> SAPAAALKKAAEAAEPATVTEDATDLQNEVDQELLKDMYGKEHVNIVFIGHVDAGKSTLGGNILFLTGMVDKRTMEKIEREAKEAGKESWYLSWALDSTSEEREKGKTVEVGRAYFETEHRRFSLLDAPGHKGYVTNMINGASQADIGVLVISARRGEFEAGFERGGQTREHAVLARTQGINHLVVVINKMDEPSVQWSEERYKECVDKLSMFLRRVAGYNSKTDVK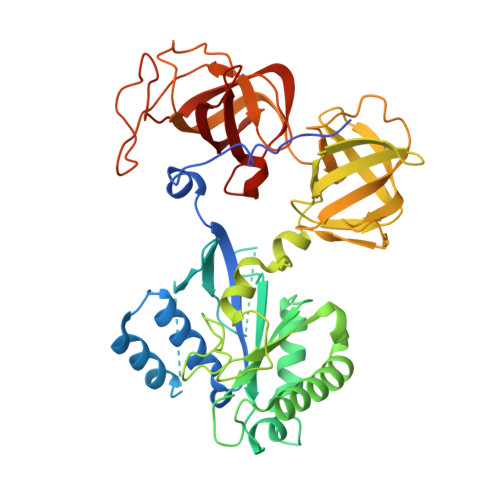YMPVSAYTGQNVKDRVDSSVCPWYQGPSLLEYLDSMTHLERKVNAPFIMPIASKYKDLGTILEGKIEAGSIKKNSNVLVMPINQTLEVTAIYDEADEEISSSICGDQVRLRVRGDDSDVQTGYVLTSTKNPVHATTRFIAQIAILELPSILTTGYSCVMHIHTAVEEVSFAKLLHKLDKTNRKSKKPPMFATKGMKIIAELETQTPVCMERFEDYQYMGRFTLRDQGTTVAVGKVVKILD>[2x]IVPDAGVGTVPMTDYGNDIEYYGQVTIGTPGKKFN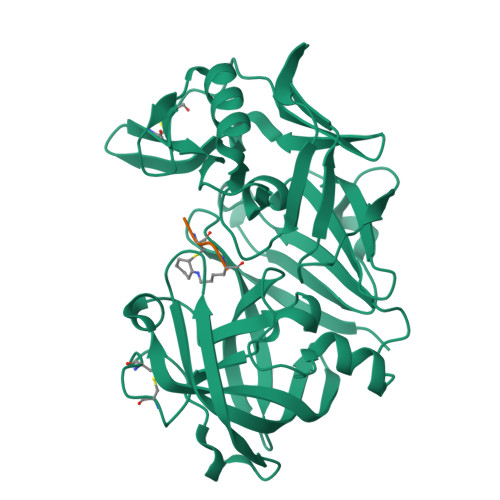LDFDTGSSDLWIASTLCTNCGSRQTKYDPNQSSTYQADGRTWSISYGDGSSASGILAKDNVNLGGLLIKGQTIELAKREAASFANGPNDGLLGLGFDTITTVRGVKTPMDNLISQGLISRPIFGVYLGKASNGGGGEYIFGGYDSTKFKGSLTTVPIDNSRGWWGITVDRATVGTSTVASSFDGILDTGTTLLILPNNVAASVARAYGASDNGDGTYTISCDTSRFKPLVFSINGASFQVSPDSLVFEEYQGQCIAGFGYGNFDFAIIGDTFLKNNYVVFNQGVPEVQIAPVAE;>[2x]ACVK>SNAAPQQINDIVHRTITPLIEQQKIPGMAVAVIYQGKPYYFTWGYADIAKKQPVTQQTLFELGSVSKTFTGVLGGDAIARGEIKLSDPTTKYWPELTAKQWNGITLLHLATYTAGGLPLQVPDEVKSSSDLLRFYQN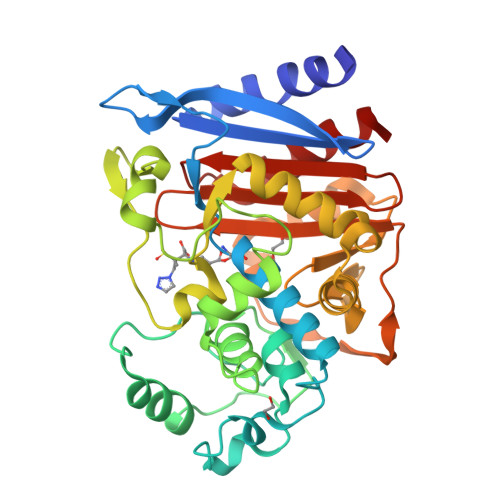WQPAWAPGTQRLYANSSIGLFGALAVKPSGLSFEQAMKTRVFQPLKLNHTWINVPSAEEKNYAWGYREGKAVHVSPGALDAEAYGVKSTIEDMARWVQSNLKPLDINEKTLQQGIQLAQSRYWQTGDMYQGLGWEMLDWPVNPDIIINGSDNKIALAARPVKPITPPTPAVRASWVHKTGATGGFGSYVAFIPEKELGIVMLANKNYPNPARVAAAWQILNALQ[4x]> GSMDPDELPLDEHCERLPYDASKWEFPRDRLKLGKPLGRGAFGQVIEADAFGIDKTATCRTVAVKMLKEGATHSEHRALMSELKILIHIGHH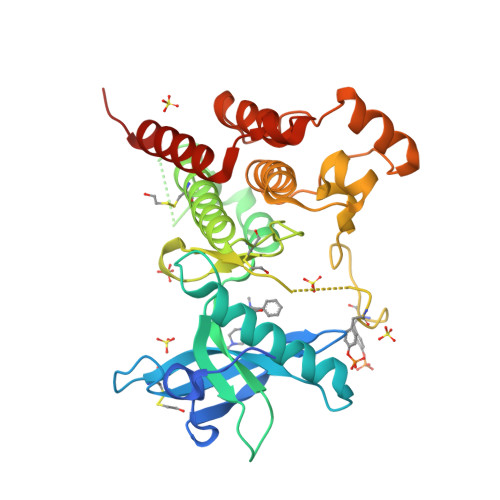LNVVNLLGACTKPGGPLMVIVEFCKFGNLSTYLRSKRNEFVPYKPEDLYKDFLTLEHLICYSFQVAKGMEFLASRKCIHRDLAARNILLSEKNVVKICDFGLARDIYKDPDYVRKGDARLPLKWMAPETIFDRVYTIQSDVWSFGVLLWEIFSLGASPYPGVKIDEEFCRRLKEGTRMRAPDYTTPEMYQTMLDCWHGEPSQRPTFSELVEHLGNLLQANAQQD> MTTLLNPYFGEFGGMYVPQILMPALNQLEEAFVSAQKDPEFQAQFADLLKNYAGRPTALTKCQNITAGTRTTLYLKREDLLHGGAHKTNQVLGQALLAKRMGKSEIIAETGAGQHGVASALASALLGLKCRIYMGAKDVERQSP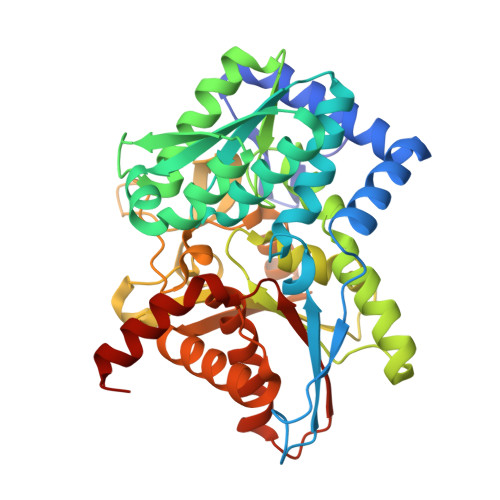NVFRMRLMGAEVIPVHSGSATLKDACNEALRDWSGSYETAHYMLGTAAGPHPYPTIVREFQRMIGEETKAQILDKEGRLPDAVIACVGGGSNAIGMFADFINDTSVGLIGVEPGGHGIETGEHGAPLKHGRVGIYFGMKAPMMQTADGQIEESYSISAGLDFPSVGPQHAYLNSIGRADYVSITDDEALEAFKTLCRHEGIIPALESSHALAHALKMMREQPEKEQLLVVNLAGRGDKDIFTVHDILKARGEI> TVESNWGGAILIGSDFDTVSATANVPSASGGSSAAGTAWVGIDGDTCQTAILQTGFDWYGDGTYDAWYEWYPEVSDDFSGITISEGDSIQMSVTATSDTSGSATLENLTTGQKVSKSFSNESSGSLCRTN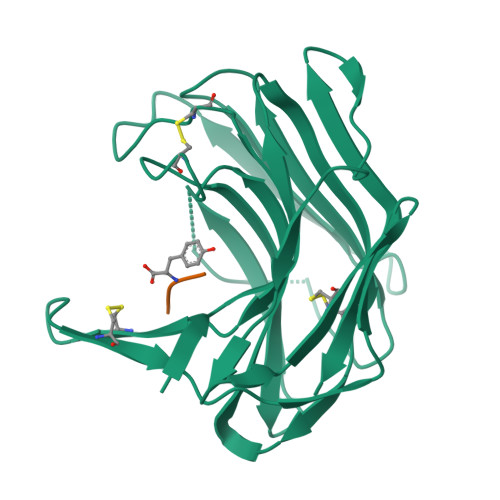AEFIIEDFEECNSNGSDCEFVPFASFSPAVEFTDCSVTSDGESVSLDDAQITQVIINNQDVTDCSVSGTTVSCSYV;> AIH> MQNSQDFSITELSLPKGGGAITGMGEALTPTGPDGMAALSLPLPISAGRGYAPAFTLNYNSGAGNSPFGLGWDCNVMTIRRRTHFGVPHYDETDTFLGPEGEVLVVADQPRDESTLQGINLGATFTVTGYRSRLESHFSRLEYWQPKTTGKTDFWLIYSPDGQVHLLGKSPQARISNPSQTTQTAQWLLEASVSSRGEQIYYQYRAEDDTGCEADEITHHLQATAQRYLHIVYYGNRTASETLPGLDGSAPSQADWLFYLVFDYGERSNNLKTPPAFSTTGSWLCRQDRFSRYEYGFEIRTRRLCRQVLMYHHLQALDSKITEHNGPTLVSRLILNYDESAIASTLVFVRRVGHEQDGNVVTLPPLELAYQDFSPRHHAHWQPMDVLANFNAIQRWQLVDLKGEGLPGLLYQDKGAWWYRSAQRLGEIGSDAVTWEKMQPLSVIPSLQSNASLVDINGDGQLDWVITGPGLRGYHSQRPDGSWTRFTPLNALPVEYTHPRAQLADLMGAGLSDLVLIGPKSVRLYANTRDGFAKGKDVVQSGDITLPVPGADPRKLVAFSDVLGSGQAHLVEVSATKVTCWPNLGRGRFGQPITLPGFSQPATEFNPAQVYLADLDGSGPTDLIYVHTNRLDIFLNKSGNGFAEPVTLRFPEGLRFDHTCQLQMADVQGLGVASLILSVPHMSPHHWRCDLTNMKPWLLNEMNNNMGVHHTLRYRSSSQFWLDEKAAALTTGQTPVCYLPFPIHTLWQTETEDEISGNKLVTTLRYARGAWDGREREFRGFGYVEQTDSHQLAQGNAPERTPPALTKNWYATGLPVIDNALSTEYWRDDQAFAGFSPRFTTWQDNKDVPLTPEDDNSRYWFNRALKGQLLRSELYGLDDSTNKHVPYTVTEFRSQVRRLQHTDSRYPVLWSSVVESRNYHYERIASDPQCSQNITLSSDRFGQPLKQLSVQYPRRQQPAINLYPDTLPDKLLANSYDDQQRQLRLTYQQSSWHHLTNNTVRVLGLPDSTRSDIFTYGAENVPAGGLNLELLSDKNSLIADDKPREYLGQQKTAYTDGQNTTPLQTPTRQALIAFTETTVFNQSTLSAFNGSIPSDKLSTTLEQAGYQQ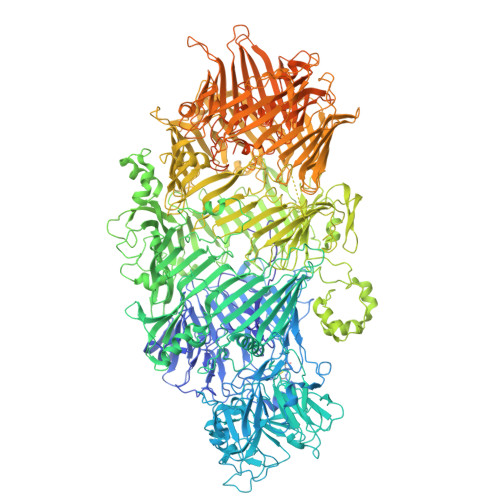TNYLFPRTGEDKVWVAHHGYTDYGTAAQFWRPQKQSNTQLTGKITLIWDANYCVVVQTRDAAGLTTSAKYDWRFLTPVQLTDINDNQHLITLDALGRPITLRFWGTENGKMTGYSSPEKASFSPPSDVNAAIELKKPLPVAQCQVYAPESWMPVLSQKTFNRLAEQDWQKLYNARIITEDGRICTLAYRRWVQSQKAIPQLISLLNNGPRLPPHSLTLTTDRYDHDPEQQIRQQVVFSDGFGRLLQAAARHEAGMARQRNEDGSLIINVQHTENRWAVTGRTEYDNKGQPIRTYQPYFLNDWRYVSNDSARQEKEAYADTHVYDPIGREIKVITAKGWFRRTLFTPWFTVNEDENDTAAEVKKVKMPGSRPMKNIDPKLYQKTPTVSVYDNRGLIIRNIDFHRTTANGDPDTRITRHQYDIHGHLNQSIDPRLYEAKQTNNTIKPNFLWQYDLTGNPLCTESIDAGRTVTLNDIEGRPLLTVTATGVIQTRQYETSSLPGRLLSVAEQTPEEKTSRITERLIWAGNTEAEKDHNLAGQCVRHYDTAGVTRLESLSLTGTVLSQSSQLLIDTQEANWTGDNETVWQNMLADDIYTTLSTFDATGALLTQTDAKGNIQRLAYDVAGQLNGSWLTLKGQTEQVIIKSLTYSAAGQKLREEHGNDVITEYSYEPETQRLIGIKTRRPSDTKVLQDLRYEYDPVGNVISIRNDAEATRFWHNQKVMPENTYTYDSLYQLISATGREMANIGQQSHQFPSPALPSDNNTYTNYTRTYTYDRGGNLTKIQHSSPATQNNYTTNITVSNRSNRAVLSTLTEDPAQVDALFDAGGHQNTLISGQNLNWNTRGELQQVTLVKRDKGANDDREWYRYSGDGRRMLKINEQQASNNAQTQRVTYLPNLELRLTQNSTATTEDLQVITVGEAGRAQVRVLHWESGKPEDIDNNQLRYSYDNLIGSSQLELDSEGQIISEEEYYPYGGTALWAARNQTEASYKTIRYSGKERDATGLYYYGYRYYQPWIGRWLSSDPAGTIDGLNLYRMVRNNPVTLLDPDGLMPEFGESLFKGPRDYNPISSTICHLTNESDGHTTSLYGIGFGPFIITNKHLFRRNNGTLLVQSLHGVFKVKNTTTLQQHLIDGRDMIIIRMPKDFPPFPQKLKFREPQREERICLVTTNFQTKSMSSMVSDTSCTFPSSDGIFWKHWIQTKDGQCGSPLVSTRDGFIVGIHSASNFTNTNNYFTSVPKNFMELLTNQEAQQWVSGWRLNADSVLWGGHKVFMVKPEEPFQPVKEATQLMNRRRRRLEHHHHHH5-(1-CARBOXY-1-PHOSPHONOOXY-ETHOXYL)-4-HYDROXY-3-PHOSPHONOOXY-CYCLOHEX-1-ENECARBOXYLIC ACID | C10 H16 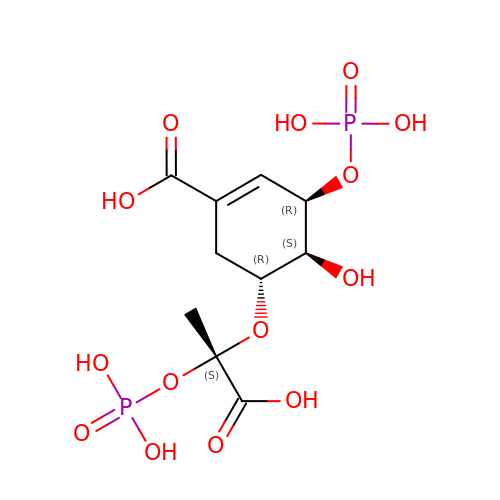O14 P2 | QUQKBSPZUVNKIF-JQCUSGDOSA-N>S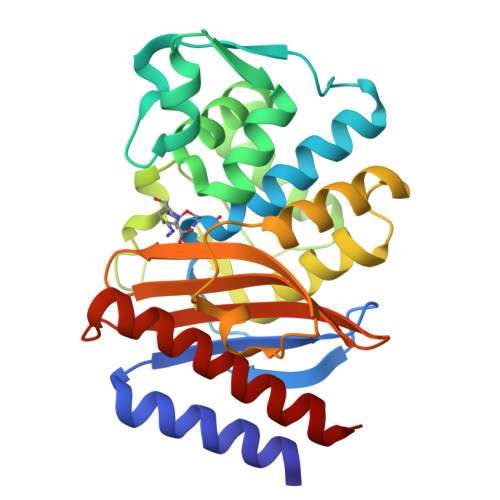EKLTFKTDLEKLEREKAAQIGVAIVDPQGEIVAGHRMAQRFAMGSTFKFPLAALVFERIDSGTERGDRKLSYGPDMIVEWSPATERFLASGHMTVLEAAQAAVQLSDNGATNLLLREIGGPAAMTQYFRKIGDSVSRLDRKEPEMSDNTPGDLRDTTTPIAMARTVAKVLYGGALTSTSTHTIERWLIGNQTGDATLRAGFPKDWVVGEKTGTCANGGRNDIGFFKAQERDYAVAVYTTAPKLSAVERDELVASVGQVITQLILSTA[2x]>[2x]MSKITKVFAREILDSRGNPTIQVDVYTLAGGFGSAIVPSGASTGSREALELRDTNTKYADNWYGQKGVMTAVDNVNNIIAPEIIGLCCKNQRLIDQKIIELDGTPNKEKLGANAILGVSLAVAKAAANELRMPLFRYLGGTNPTLMPVPMLNVINGGEHASNTLDFQEFMIMPLGFRTFKEALQAANKVFHNLAKLLKKSGFETQVGDEGGFAPNFNSHEQALDFLVDAIKESG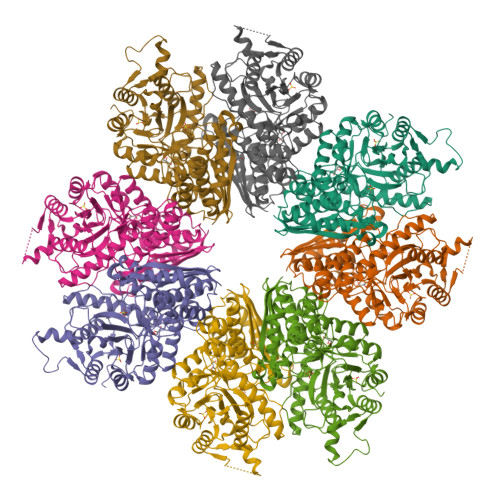FNPGFKGENAVAIAIDAAASEFYNGQKYVFKKLKAASLSKNQADLDEKFEFNSEELLNYYGQLLAKYPIISIEDGFAESDWQGFIAFNQKYGNNHQIVGDDLTVTNVEILKKAINLKAINSILIKLNQIGTLSETLDAIHLAQKSGMTAVISHRSGESEDTTIADLAVAVSSGQIKTGSLSRTDRIAKYNRLLVIEEYLNSYAKADYIGREVFYNLKKLEHHHHHH> MKNLKSNDVLLHSVTRVVTFIILAFSVYLFFAGHNNPGGGFIGGLMTASALLLMYLGFDMKSIKKAIPFDFTKMIAFGL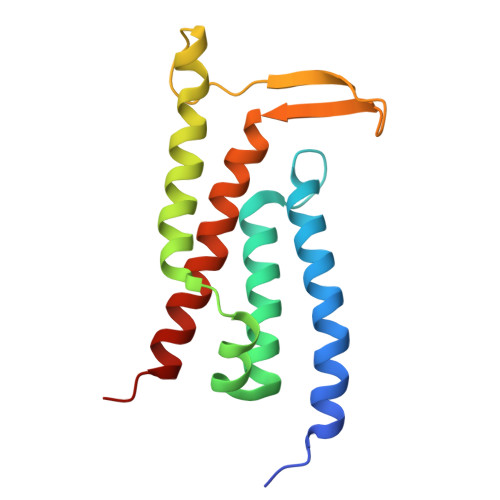LLAIITGFGGLLVGDPYLTQYFEYYQIPILGETELTTALPFDLGIYLVVVGIALTIILTIAEDDM>[4x]GSMKPYKELERVFTKLYRYGHMLLLADWDSHTMMPCKGSDARGAAMAELQLHMHDTITAPKIRALIEEAEKSVGDLEKLQRANLREMRRAWELENLLPEEFVERKTVLTTKAHQVWKTCREKNDFAGFLPTLKELIALFREEGKLRAGNSGKHPYEALVDIYEPGMTLQRLDEIFGNVRSWLPELLKEVQEKQKALGETVLEPKGPFPVSKQEALCRFFMDVWKFDFDGGRLDVSAHP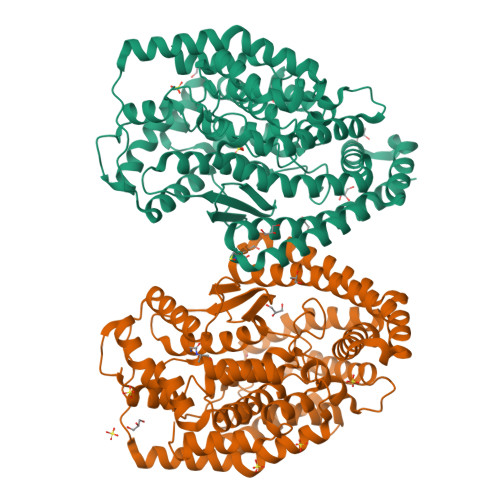FCGNSKEDVRITTKYTETEFVTSLLGVIHETGHAKYEQNCGPKGFETQPVCMARSLGVHEGQSLFAEMQIGRSGAFMEFLAPRLVEYFGDQPAFTSSNMKRVIQRVSPGLIRIDADELCYPLHVMLRYEIERDLMDGNIEAEEVPRVWNEKMKSYLGLETLGNDKEGCLQDVHWSGGMFGYFPTYSLGAMVAAQLMSCVRRELGEEVVDDCIRKGDLGKILAKQNEKIWQHGSSLTTDELLRQATGETLNPEHYRRHLERRYRDDRG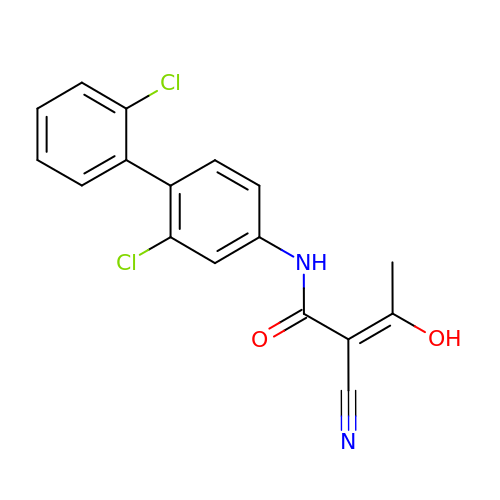(2Z)-2-cyano-N-(2,2'-dichlorobiphenyl-4-yl)-3-hydroxybut-2-enamide | C17 H12 Cl2 N2 O2 | DDSLONVJHZPSBB-UVTDQMKNSA-N> EPCVEVVPNITYQCMELNFYKIPDNLPFSTKNLDLSFNPLRHLGSYSFFSFPELQVLDLSRCEIQTIEDGAYQSLSHLSTLILTGNPIQSLALGAFSGLSSLQKLVAVETNLASLENFPIGHLKTLKELNVAHNLIQSFKLPEYFSNLTNLEHLDLSSNKIQSIYCTDLRVL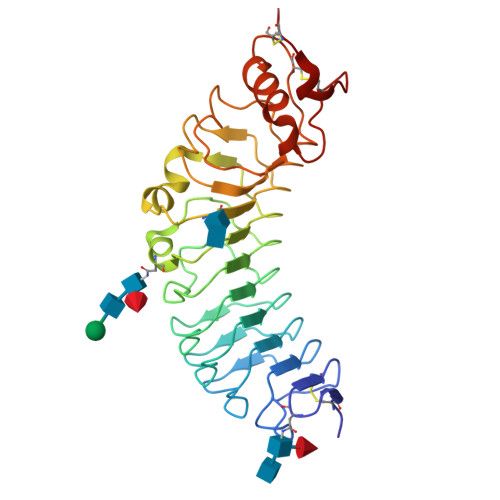HQMPLLNLSLDLSLNPMNFIQPGAFKEIRLKELALDTNQLKSVPDGIFDRLTSLQKIWLHTNPWDCSCPRIDYLSRWLNKNSQKEQGSAKCSGSGKPVRSIICP>[2x]APLAQPELCAVDTAPGYVAGAHQFGLSQNSHLVLPLQQSDVRKRLQVQLSIRTFASSGLIYYVAHQNQMDYATLQLQEGRLHFMFDLGKGRTKVSHPALLSDGKWHTVKTEYIKRKAFMTVDGQESPSVTVVGKATTLD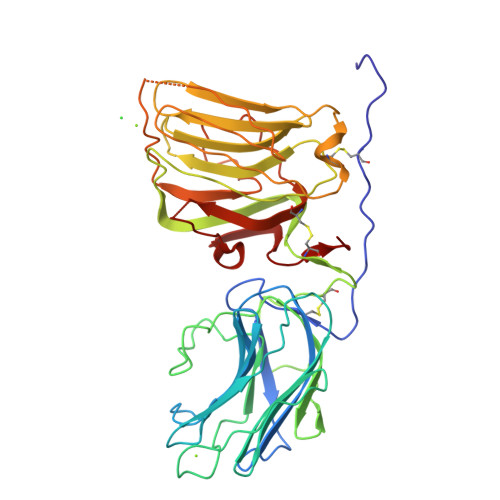VERKLYLGGLPSHYRARNIGTITHSIPACIGEIMVNGQQLDKDRPLSASAVDRCYVVAQEGTFFEGSGYAALVKEGYKVRLDLQITLEFRTTSKNGVLLGISSAKVDAIGLEIVDGKVLFHVNNGAGRITATYQPRAARALCDGKWHTLQAHKSKHRIVLTVDGNSVRAESPHTHSTSADTNDPIYVGGYPAHIKQNSLSSRASFRGCVRNLRLSRGSQVQSLDLSRAFDLQGVFPHSCPGPEP> FDRDRLFSVVSRGVPEELTGLLEYLRWNSKYLTDSAYTEGSTGKTCLMKAVLNLQDGVNACIMPLLQIDKDSGNPKPLVNAQCTDEFYQGHSALHIAIEKRSLQCVKLL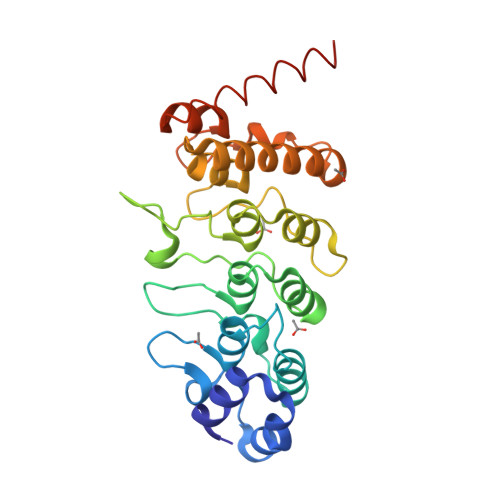VENGADVHLRACGRFFQKHQGTCFYFGELPLSLAACTKQWDVVTYLLENPHQPASLEATDSLGNTVLHALVMIADNSPENSALVIHMYDGLLQMGARLCPTVQLEEISNHQGLTPLKLAAKEGKIEIFRHILQREFSGAAAHHHHHH>[3x]AMSTQGLVQLLANAQCHLRTSTNYNGVHTQFNSALNYKNNGTNTIDGSEAWCSSIVDTNQYIVAGCEVPRTFMCVALQGRGDADQWVTSYKIRYSLDNVSWFEYRNGAAVTGVTDRNTVVNHFFDTPIR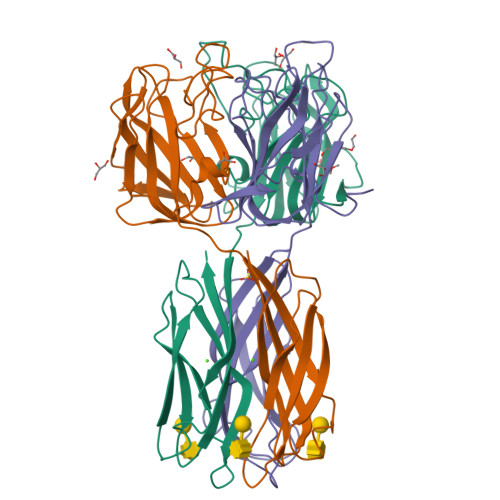ARSIAIHPLTWNGHISLRCEFYTQPVQSSVTQVGADIYTGDNCALNTGSGKREVVVPVKFQFEFATLPKVALNFDQIDCTDATNQTRIGVQPRNITTKGFDCVFYTWNENKVYSLRADYIATALE> MAKLTALTLLGMGLALFDRQKSSFQTRFNVHREVTPVELPNCNLVKGIDNGSEDLEILPNGLAFISSGSKYPGIMSFDPDKSGKILLMDLNEKEPAVSELEIIGNTLDISSFNPWGISTFIDDDNTVYLLVVNHPGSSSTVEVFKFQEEEKSLLHLKTIRHKLLPSVNDIVAVGPEHFYATNDHYFIDP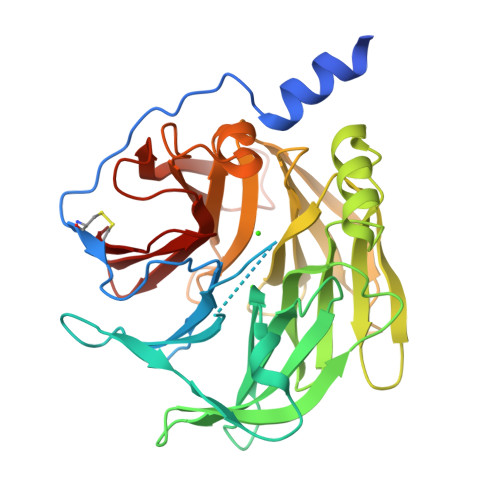YLKSWEMHLGLAWSFVTYYSPNDVRVVAEGFDSANGINISPDGKYVYIAELLAHKIHVYEKHANWTLTPLRVLSFDTLVDNISVDPVTGDLWVGCHPNGMRIFFYDAENPPGSEVLRIQDILSEEPKVTVVYAENGTVLQGSTVAAVYKGKLLIGTVFHKALYCDL> CYFQNC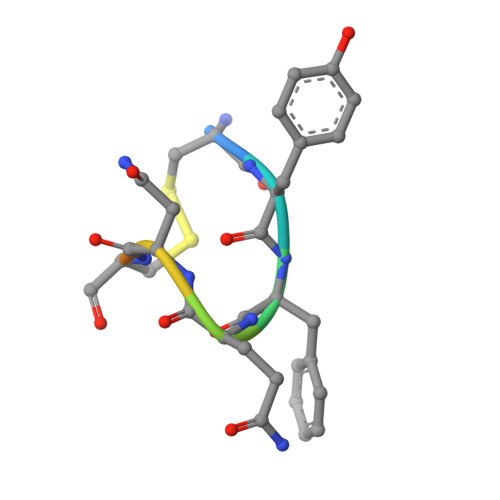PKG> MAQFAFESDLHSLLQLDAPIPNAPPARWQRKAKEAAGPAPSPMRAANRSHSAG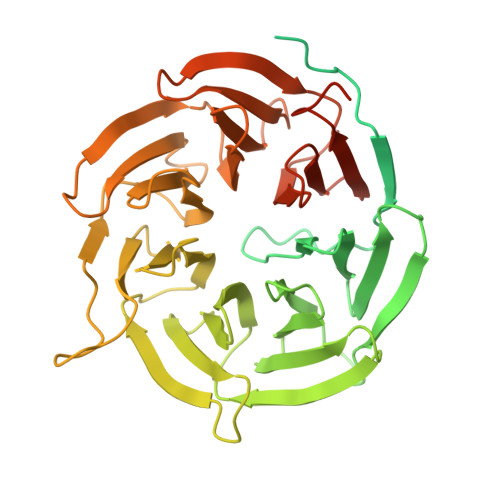RTPGRTPGKSSSKVQTTPSKPGGDRYIPHRSAAQMEVASFLLSKENQPENSQTPTKKEHQKAWALNLNGFDVEEAKILRLSGKPQNAPEGYQNRLKVLYSQKATPGSSRKTCRYIPSLPDRILDAPEIRNDYYLNLVDWSSGNVLAVALDNSVYLWSASSGDILQLLQMEQPGEYISSVAWIKEGNYLAVGTSSAEVQLWDVQQQKRLRNMTSHSARVGSLSWNSYILSSGSRSGHIHHHDVRVAEHHVATLSGHSQEVCGLRWAPDGRHLASGGNDNLVNVWPSAPGEGGWVPLQTFTQHQGAVKAVAWCPWQSNVLATGGGTSDRHIRIWNVCSGACLSAVDAHSQVCSILWSPHYKELISGHGFAQNQLVIWKYPTMAKVAELKGHTSRVLSLTMSPDGATVASAAADETLRLWRCFELDPARRREREKASAAKSSLIHQGIR2,4-dichlorophenol | C6 H4 Cl2 O 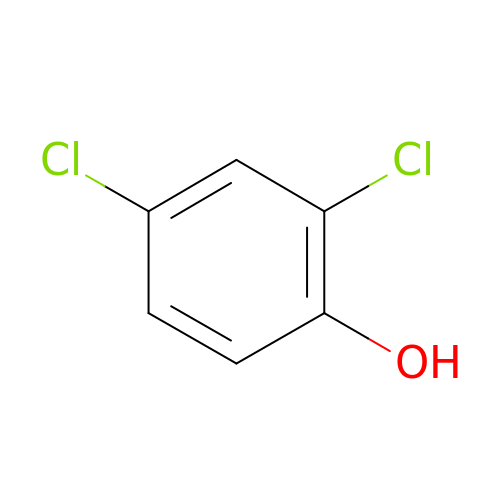| HFZWRUODUSTPEG-UHFFFAOYSA-N> GKSAVIFVERATPATLTELKDALSNSILSVRDPWSIDFRTYRCSIKNLPADVSKLMYSITFHHHGRQTVLIKDNSAMVTTAAAA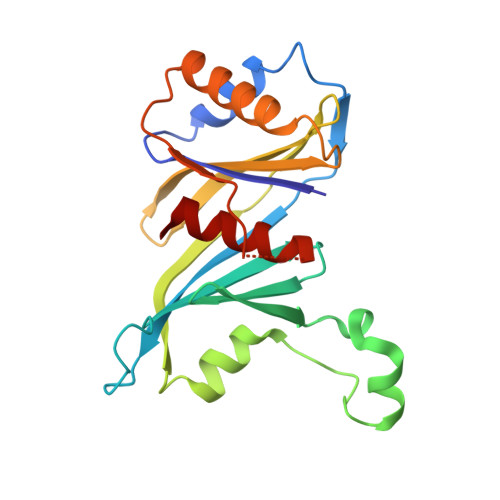DIPPALVFNGSSTGVPESIDTILSSKLSNIWMQRQLIKGDAGETLILDGLTVRLVNLFSSTGFKGLLIELQADEAGEFETKIAGIEGHLAEIRAKEYKTSSDSLGPDTSNEICDLAYQYVRALEL>MHHHHHHMTKQALLEVSNLVREFPAGESTIQILKGIDLTIYEGELVAIVGQSGSGKSTLMNILGCLDRPTSGSYKVNGQETGKLEPDQLAQLRREYFGFIFQRYHLLGDLSAEGNVEVPAVYAGVTPADRKQRATALLTELGLGTKTQNRPSQLSGGQQQRVSIARALMNGGDVILADEPTGALDSHSGVEVMRILRELNAAGHTIILVTHDMQVAKNATRIIEISDGEIISDRPNVPDQSLEEVKSDPDAAPALQNKQKKGKSISAWRSTLDRLSEAFQMALLSMNAHRMRTFLTMLGIIIGIASVVTVVALGNGSQQQILSNISSLGTNTITVFQGRGFGDNSKTANFKTLVPADADALMTQPYVSAVSPMVSTSKTMRYQQNEANATINGVSNDYFDVKGLVFKDGQTFDQRSVRDRSQDVVIDTNTQKQFFSDGTNPIGQVVLLGSVPARIIGIVEPQTSGMGSDDTLNVYMPYTTVMSRMLGQAHVRNIVVRINDKYSTSAAENAIVNLLTQRHGAQDIFTMNSDSIRQTIEKTTSTMTLLVSAIAVISLVVGGIGVMNIMLVSVTERTQEIGVRMAVGARQSDILQQFLIEAILVCLIGGVLGVLLSLGLGQLINKFAGGNFAVAYSTTSIVAAFVCSTLIGVVFGFLPA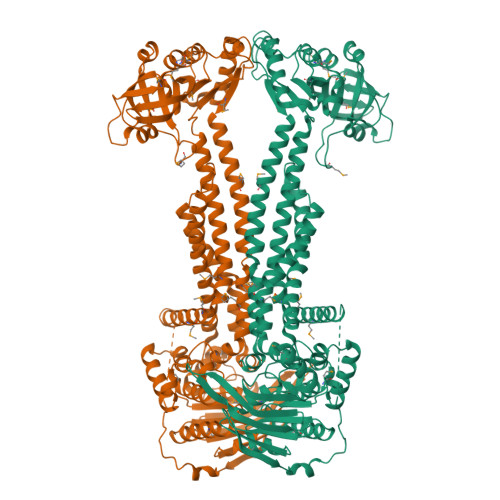KNAAKLDPVAALSRE[2x]>SNAMKRAVITGLGIVSSIGNNQQEVLASLQEGRSGITFAQEFKDAGMRSHVWGDVKLQSEPKDLIDRKVLRFMSDASIYAYLAMQEAIADSGLSDSQVSNFRSGLVVGSGGGSPRNQVAGSDAMRTPRGLKGVGPYMVTKAMASGVSACLATPFKIKGVNYSISSACATSAHCIGHALELIQLGKQDIVFAGGGEELCWEMACEFDAMGALSTKYNDTPAKASRTYDQDR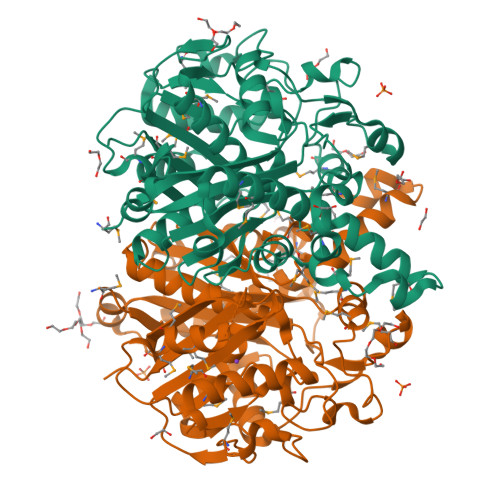DGFVIAGGGGMVVVEELEHALARGAHIYAEIVGYGATSDGADMVAPSGEGAVRCMQMAMAGVDTPIDYMNVHGTSTPVGDVKELGAIREVFGNNTPAISSTKAMTGHSLGAAGVHEAIFSLLMVEHGFIAPSINIDNLDEQAQGMNIITETTQRELTTVMSNSFGFGGTNATLVMRKYQK[2x]2-[({2-[(3s,5s,7s)-tricyclo[3.3.1.1~3,7~]dec-1-yl]ethyl}amino)methyl]phenol | C19 H27 N O | 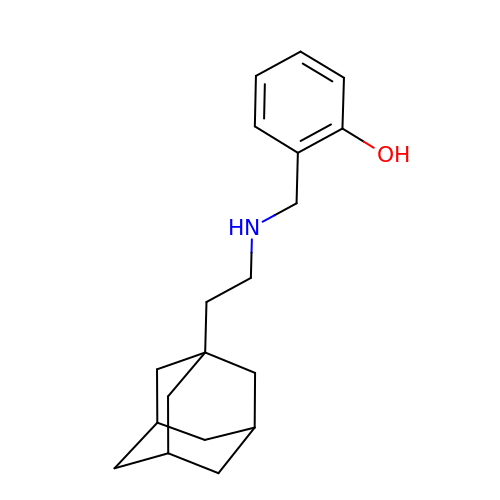ZQPUAJLAXSAIEG-IAKCYEPBSA-N>[22x]MDLLTAKTIVLG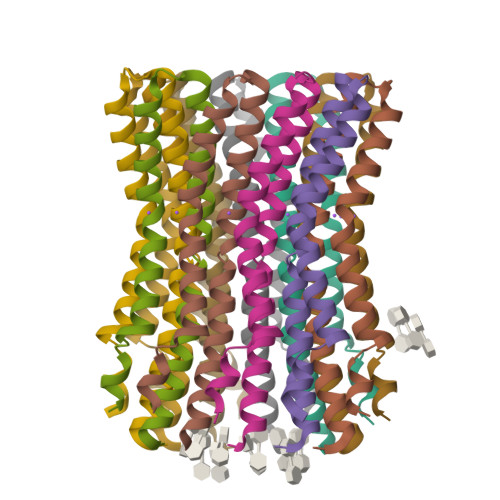CSAVGAGLAMIAGLGPGIGEGYAAGKAVESVARQPEARGSIISTMILGQAVAESTGIYSLVIALILLYANPFLSKLG>[2x]SHMTMEQFLTSLDMIRSGCAPKFKLKTEDLDRLRVGDFNFPPSQDLMCY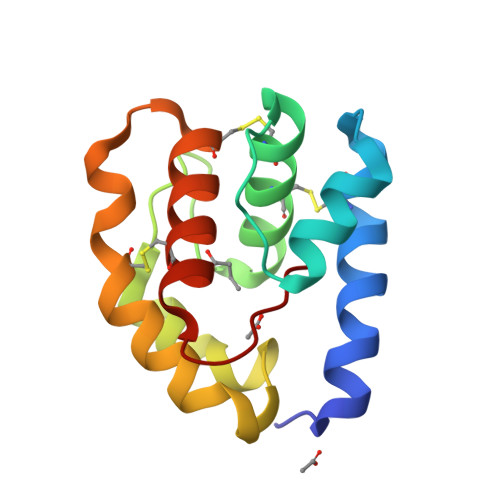TKCVSLMAGTVNKKGEFNAPKALAQLPHLVPPEMMEMSRKSVEACRDTHKQFKESCERVYQTAKCFSENADGQFMWP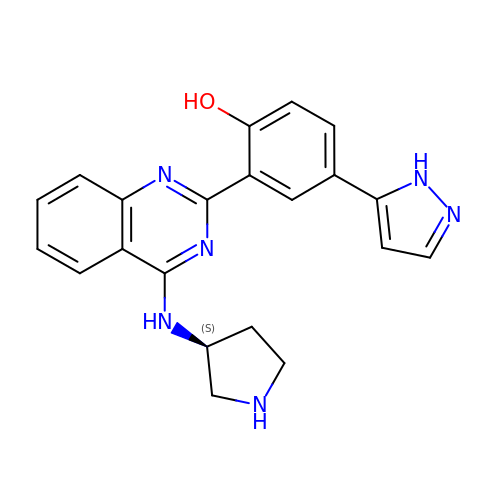4-(1H-pyrazol-5-yl)-2-{4-[(3S)-pyrrolidin-3-ylamino]quinazolin-2-yl}phenol | C21 H20 N6 O | DZNFGQDAMCNMLC-AWEZNQCLSA-N> MYIVVVYDVGVE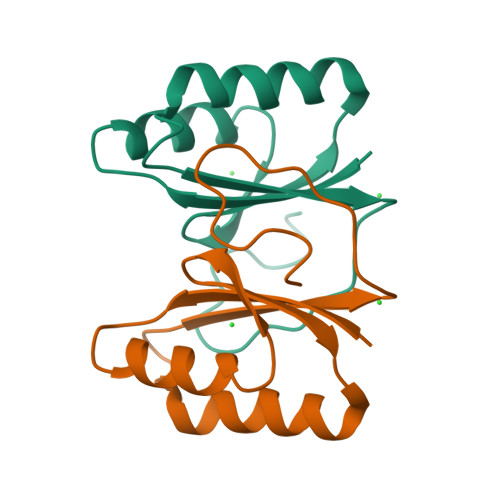RVNKVKKFLRMHLNWVQNSVFEGEVTLAEFERIKEGLKKIIDENSDSVIIYKLRSMPPRETLGIEKNPIEEII~{N}-[(1-ethyl-4-methyl-2-oxidanylidene-quinolin-6-yl)methyl]benzenesulfonamide 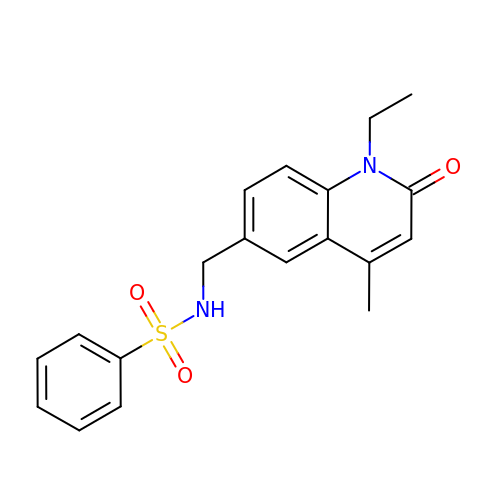| C19 H20 N2 O3 S | ZRTFSGAREQNMFJ-UHFFFAOYSA-N5-[3-[bis(oxidanyl)-$l^{3}-sulfanyl]oxy-4-chloranyl-phenyl]-~{N}-(4-piperazin-1-ylphenyl)-~{N}-(pyridin-2-ylmethyl)furan-2-carboxamide | C27 H27 Cl N4 O6 S | 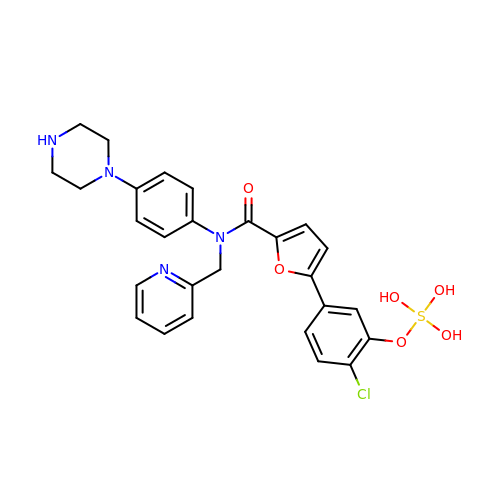OYYFNINEAKHFQQ-UHFFFAOYSA-N> MTEKEEKEDLQAQDKEEQQIKADTKVISVQEFEEYMRFKEQANSKSKETSRDLSINERITKELAEVEERERI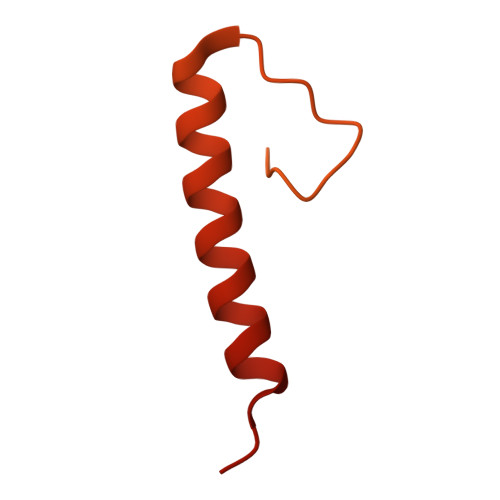EKQLLLEAERINEIDTLAKAHLSNHFNKEVLLAKGYTLKDIMQAQRRELVRKFVPIEQIKAIAKVSDISHIDGEILEQLVSLAKVNIKLRKNASSSSSSVDSIKGNIAIKSEERASLLDSNFVPINFTEFVQAISNTYKQRRIQFYENLKRHKRTSIA>KVVKFSYMWTINNFSFCREEMGEVIKSSTFSSGANDKLKWCLRVNPKGLDEESKDYLSLYLLLVSCPKSEVRAKFKFSILNAKGEETKAMESQRAYRFVQGKDWGFKKFIRRDFLLDEANGLLPDDKLTLFCEVSVVQD[2x];>[2x]EVSIIQGA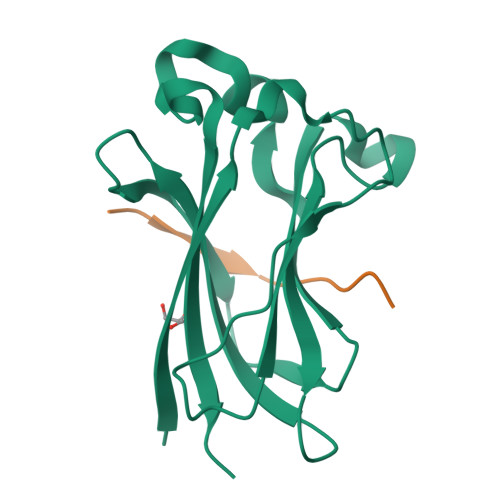DSTT>MNATINDDDIDDVKKALDHATQAAHKAAAELTAKLRSDFVEYGNGGTAGQVLIHIYGPGLIYGFSAFPVQIRLEIPNQPVPFNKVHITEVTAYVIDENNRTYWTRVWNSSTFRQGGYIADTLDLVTVMKAPDPLVYQIRDAIVTGQISRELYDKIWNTSTTHFEIRVIVKGYQEAWKTDSSVSNQSSCPSDGHWYEDACWVHDKDIDFTLKAETTTAWGHVTGTNDVATIDGGMLGSLPIKFLQSLDLSGKWVLYQNKYAGALSDFIIITAASPVHVLNSTAMYKFLITPNPGYFQPANPKISDEYRFVTLRVIEGGRMELADTTTGHIGDLTEPTFFGLTAHYTDAPGTLDYHALGLVYAYVERDDGVKIPIWLAAEPMISVLSNTYTVMKDQDVKNLIDLYKKKDREKINATTKAMINSLQEKI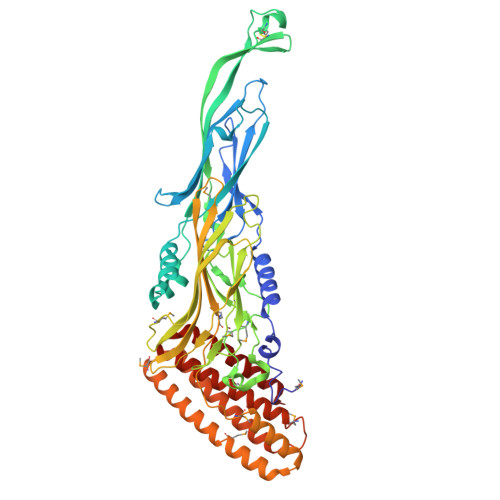DEAEQLLAKAKGMNNENAIEYAQGAIDEYKAAINDLQKAAQQDDYQMFLNYLNAAKKHEMAGDYYVNAARKALNGDLEQAKIDAEKAKEYSNLAKEYEPG[2x]> MSEFLTPERTVYDSGVQFLRPKSLDEFIGQENVKKKLSLALEAAKMRGEVLDHVLLAGPPGLGKTTLAHIIASELQTNIHVTSGPVLVKQGDMAAILTSLERGDVLFIDEIHRLNKAVEELLYSAIEDFQIDIMIGKGPSAKSIRIDIQPFTLVGATTRSGLLSSPLRSRFGIILELDFYTVKEL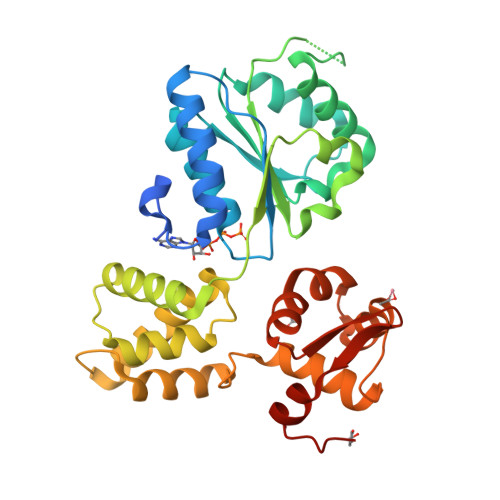KEIIKRAASLMDVEIEDAAAEMIAKRSRGTGRIAIRLTKRVRDMLTVVKADRINTDIVLKTMEVLNIDDEGLDEFDRKILKTIIEIYRGGPVGLNALAASLGVEADTLSEVYEPYLLQAGFLARTPRGRIVTEKAYKHLKYEVPENRLF> MSKTVEDRAAQRAKGPATVLAIGTATPANVVYQTDYPDYYFRVTKSEHMTKLKNKFQRMCDRSTIKKRYMVLTEELLEKNLSLCTYMEPSLDARQDILVPEVPKLGKEAADEAIAEWGRPKSEITHLIFCTTCGVDMPGADYQLTKLLGLRSSVRRTMLYQQGCFGGGTVLRLAKDLAEN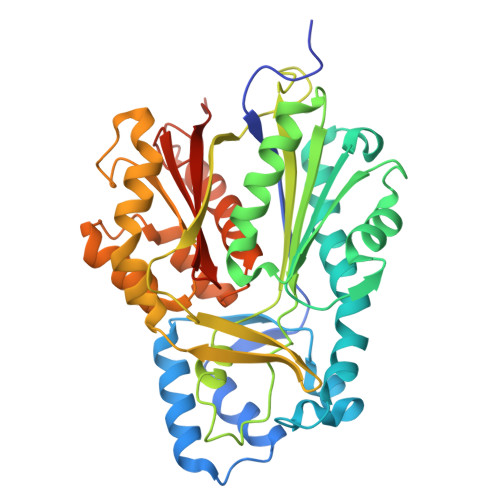NAGARVLVVCSEITTAVNFRGPSDTHLDLLVGLALFGDGAAAVIVGADPDPTLERPLFQIVSGAQTILPDSEGAINGHLREVGLTIRLLKDVPGLVSMNIEKCLMEAFAPMGIHDWNSIFWIAHPGGPTILDQVEAKLGLKEEKLKSTRAVLREYGNMSSACVLFILDEVRKRSMEEGKTTTGEGFDWGVLFGFGPGFTVETVVLHSMPIPKADEGR>HHHHHHSSGLVPRGSHMQFVNKQFNYKDPVNGVDIAYIKIPNVGQMQPVKAFKIHNKIWVIPERDTFTNPEEGDLNPPPEAKQVPVSYYDSTYLSTDNEKDNYLKGVTKLFERIYSTDLGRMLLTSIVRGIPFWGGSTIDTELKVIDTNCINVIQPDGSYRSEELNLVIIGPSADIIQFECKSFGHEVLNLTRNGYGSTQYIRFSPDFTFGFEESLEVDTNPLLGAGKFATDPAVTLAHELIHAGHRLYGIAINPNRVFKVNTNAYYEMSGLEVSFEELRTFGGHDAKFIDSLQENEFRLYYYNKFKDIASTLNKAKSIVGTTASLQYMKNVFKEKYLLSEDTSGKFSVDKLKFDKLYKMLTEIYTEDNFVKFFKVLNRKTYLNFDKAVFKINIVPKVNYTIYDGFNLRNTNLAANFNGQNTE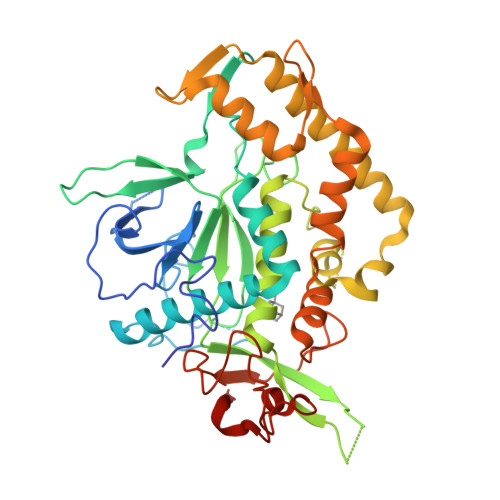INNMNFTKLKNFTGLFEF[2x]> HMPSFDFDIPRRSPQEIAKGMVAIPGGTFRMGGEDPDAFPEDGEGPVRTVRLSPFLIDRYAVSNRQFAAFVKATGYVTDAERYGWSFVFHAHVAPGTPVMDAVVPEAPWWVAVPGAYWKAPEGPGSSITDRPNHPV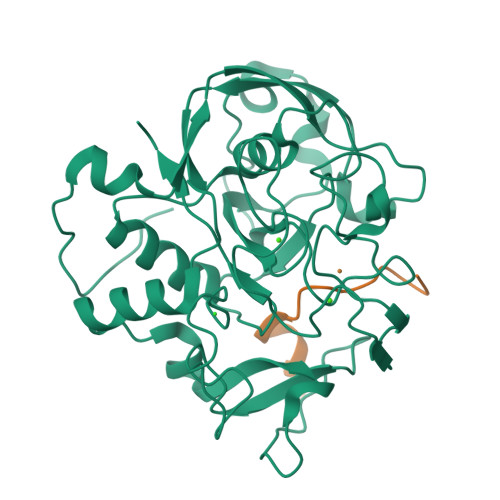VHVSWNDAVAYATWAGKRLPTEAEWEMAARGGLDQARYPWGNELTPRGRHRCNIWQGTFPVHDTGEDGYTGTAPVNAFAPNGYGLYNVAGNVWEWCADWWSADWHATESPATRIDPRGPETGTARVTKGGSFLCHESYCNRYRVAARTCNTPDSSAAHTGFRCAADP;> XATTPLCGPSRASILSG>[180x]ANKPMQPITSTANKIVWSDPTRLSTTFSASLLRQRVKVGIAELNNVSGQYVSVYKRPAPKPEGCADACVIMPN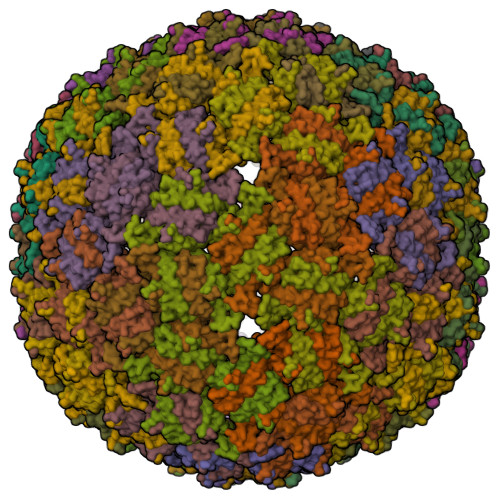ENQSIRTVISGSAENLATLKAEWETHKRNVDTLFASGNAGLGFLDPTAAIVSSDTT> GMSDVAETLDPLRLPLQGERLIEASAGTGKTFTIAALYLRLLLGLGGSAAFPRPLTVEELLVVTFTEAATAELRGRIRSNIHELRIACLRETTDNPLYERLLEEIDDKAQAAQWLLLAERQMDEAAVFTIHGFCQRMLNLNAFESGMLFEQQLIEDESLLRYQACADFWRRHCYPLPREIAQVVFETWKGPQALLRDINRYLQGEAPVIKAPPPDDETLASRHAQIVARIDTVKQQWRDAVGELDALIESSGIDRRKFNRSNQAKWIDKISAWAEEETNSYQLPESLEKFSQRFLEDRTKAGGETPRHPLFEAIDQLLAEPLSIRDLVITRALAEIRETVAREKRRRGELGFDDMLSRLDSALRSESGEVLAAAIRTRFPVAMIDEFQDTDPQQYRIFRRIWHHQPETALLLIGDPKQAIYAFRGADIFTYMKARSEVHAHYTLDTNWRSAPGMVNSVNKLFSQTDDAFMFREIPFIPVKSAGKNQALRFVFKGETQPAMKMWLMEGESCGVGDYQSTMAQVCAAQIRDWL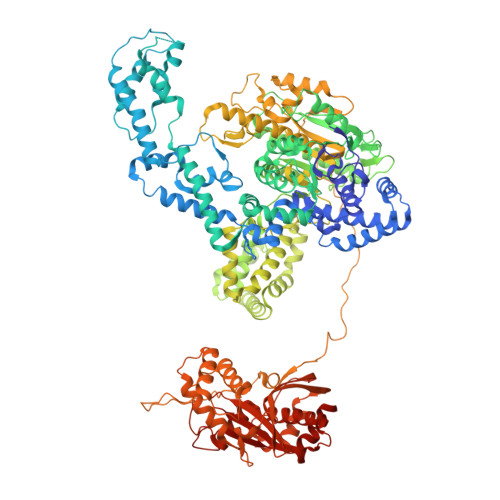QAGQRGEALLMNGDDARPVRASDISVLVRSRQEAAQVRDALTLLEIPSVYLSNRDSVFETLEAQEMLWLLQAVMTPERENTLRSALATSMMGLNALDIETLNNDEHAWDVVVEEFDGYRQIWRKRGVMPMLRALMSARNIAENLLATAGGERRLTDILHISELLQEAGTQLESEHALVRWLSQHILEPDSNASSQQMRLESDKHLVQIVTIHKSKGLEYPLVWLPFITNFRVQEQAFYHDRHSFEAVLDLNAAPESVDLAEAERLAEDLRLLYVALTRSVWHCSLGVAPLVRRRGDKKGDTDVHQSALGRLLQKGEPQDAAGLRTCIEALCDDDIAWQTAQTGDNQPWQVNDVSTAELNAKTLQRLPGDNWRVTSYSGLQQRXXXXXXXXXXXXXXXXXXXXXXXXXPTLTPHQFPRGASPGTFLHSLFEDLDFTQPVDPNWVREKLELGGFESQWEPVLTEWITAVLQAPLNETGVSLSQLSARNKQVEMEFYLPISEPLIASQLDTLIRQFDPLSAGCPPLEFMQVRGMLKGFIDLVFRHEGRYYLLAYKSNWLGEDSSAYTQQAMAAAMQAHRYDLQYQLYTLALHRYLRHRIADYDYEHHFGGVIYLFLRGVDKEHPQQGIYTTRPNAGLIALMDEMFAGMTLEEA>MGHHHHHHHHHHSSGHIDDDDKHMHNDKDLSTWQTFRRLWPTIAPFKAGLIVAGVALILNAASDTFMLSLLKPLLDDGFGKTDRSVLVWMPLVVIGLMILRGITSYVSSYCISWVSGKVVMTMRRRLFGHMMGMPVSFFDKQSTGTLLSRITYDSEQVASSSSGALITVVREGASIIGLFIMMFYYSWQLSIILIVLAPIVSIAIRVVSKRFRNISKNMQNTMGQVTTSAEQMLKGHKEVLIFGGQEVETKRFDKVSNRMRLQGMKMVSASSISDPIIQLIASLALAFVLYAASFPSVMDSLTAGTITVVFSSMIALMRPLKSLTNVNAQFQRGMAACQTLFTILDSEQEKDEGKRVIERATGDVEFRNVTFTYPGRDVPALRNINLKIPAGKTVALVGRSGSGKSTIASLITRFYDIDEGEILMDGHDLREYTLASLRNQVALVSQNVHLFNDTVANNIAYARTEQYSREQIEEAARMAYAMDFINKMDNGLDTVIGENGVLLSGGQRQRIAIARALLRDSPILILDEATSALDTESERAIQAALDELQKNRTSLVIAHRL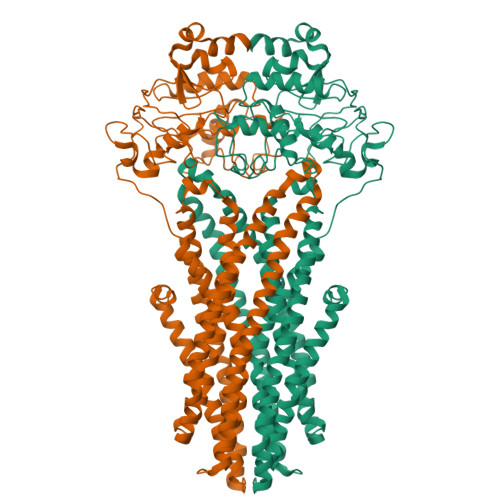STIEKADEIVVVEDGVIVERGTHNDLLEHRGVYAQLHKMQFGQ[2x]>[2x]TGQDALVLGFDWGKFLKDHSYKAAPVSCFKHVPLYDQWEDVMKGMKVEVLNSDAVLPSRV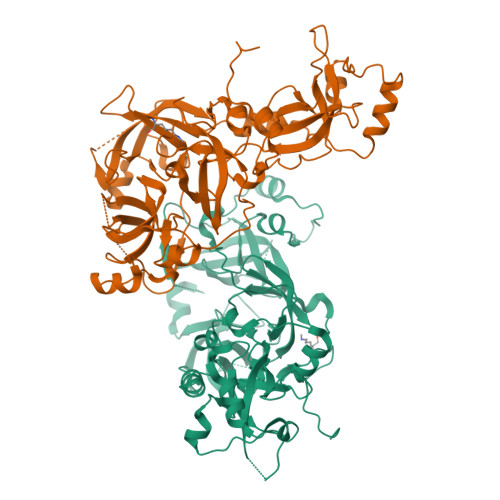YWIASVIQTAGYRVLLRYEGFENDASHDFWCNLGTVDVHPIGWCAINSKILVPPRTIHAKFTDWKGYLMKRLVGSRTLPVDFHIKMVESMKYPFRQGMRLEVVDKSQVSRTRMAVVDTVIGGRLRLLYEDGDSDDDFWCHMWSPLIHPVGWSRRVGHGIKMSERRSDMAHHPTFRKIYCDAVPYLFKKVRAVYTEGGWFEEGMKLEAIDPLNLGNICVATVCKVLLDGYLMICVDGGPSTDGLDWFCYHASSHAIFPATFCQKNDIELTPPKGYEAQTFNWENYLEKTKSKAAPSRLFNMDCPNHGFKVGMKLEAVDLMEPRLICVATVKRVVHRLLSIHFDGWDSEYDQWVDCESPDIYPVGWCELTGYQLQPPVAAEPATPLKAKEATKKKKKQ>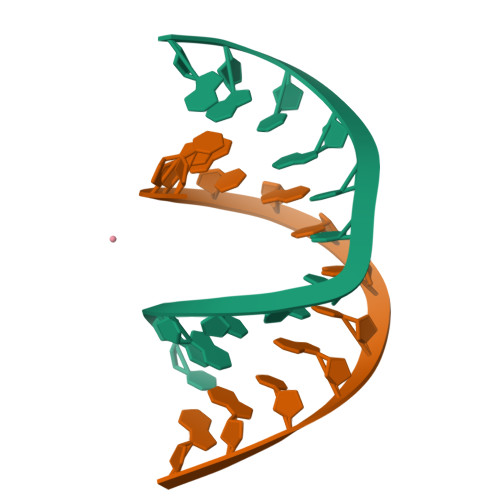[2x]CTACGTACGTAG>GSHMGRRKRTAVTGSQTALLLRAFEKDRFPGIAAREELARETGLP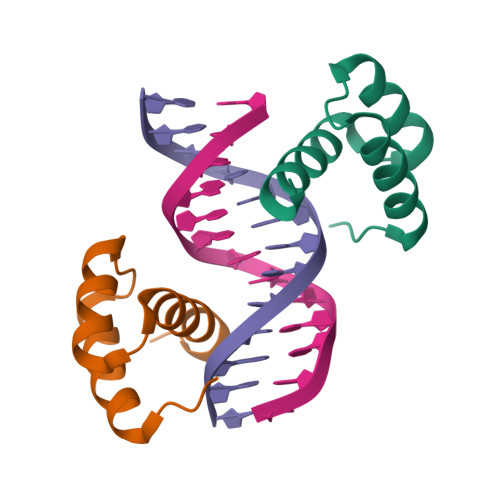ESRIQIWFQNRRARHPGQG[2x]(3S)-3-benzyl-3-methyl-5-[5-(2-methylpyrimidin-5-yl)pyrazolo[1,5-a]pyrimidin-3-yl]-1,3-dihydro-2H-indol-2-one 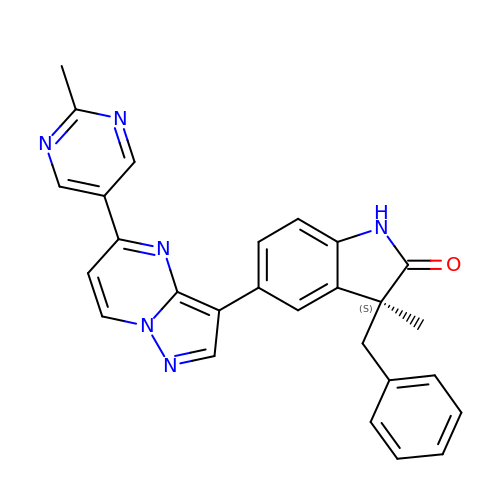| C27 H22 N6 O | KQGDDLRQLMABOG-MHZLTWQESA-N> MKAPAFTEAKLQDPIPAKIYDKNGELVKTLDNGQRHEHVNLKDVPKSMKDAVLATEDNRFYEHGALDYKRLFGAIGKNLTGGFGSEGASTLTQQVVKDAFLSQHKSIGRKAQEAYLSYRLEQEYSKDDIFQVYLNKIYYSDGVTGIKAAAKYYFNKDLKDLNLAEEAYLAGLPQVPNNYNIYDHPKAAEDRKNTVLYLMHYHKRITDKQWEDAKKIDLKANLVNRTPEERQNIDTNQDSEYNSYVNFVKSELMNNKAFKDENLGNVLQSGIKIYTNMDKDVQKTLQNDVDNGSFYKNKDQQVGATILDSKTGGLVAISGGRDFKDVVN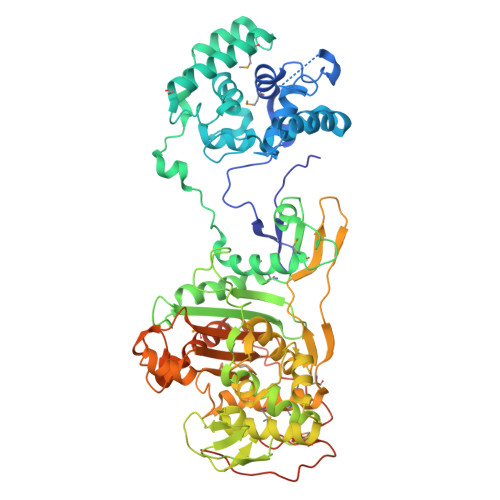RNQATDPHPTGSSLKPFLAYGPAIENMKWATNHAIQDESSYQVDGSTFRNYDTKSHGTVSIYDALRQSFNIPALKAWQSVKQNAGNDAPKKFAAKLGLNYEGDIGPSEVLGGSASEFSPTQLASAFAAIANGGTYNNAHSIQKVVTRDGETIEYDHTSHKAMSDYTAYMLAEMLKGTFKPYGSAYGHGVSGVNMGAKTGTGTYGAETYSQYNLPDNAAKDVWINGFTPQYTMSVWMGFSKVKQYGENSFVGHSQQEYPQFLYENVMSKISSRDGEDFKRPSSVSGSIPSINVSGSQDNNTTNRSTHGGSDTSANSSGTAQSNNNTRSQQSRNSGGLTGIFN> MTTLRAFTCDDLFRFNNINLDPLTETYGIPFYLQYLAHWPEYFIVAEAPGGELMGYIMGKAEGSVAREEWHGHVTALSVAPEFRRLGLAAKLMELLEEISERKGGFFVDLFVRVSNQVAVNMYKQLGYSVYRTVIEYYSASNGEPDEDAYDMRKALSRDTEKK;> MATRGHVQDPNDRRLRPIYDYLDNGNNKMAIQQADKLLKKHKDLHCAKVLKAIGLQRTGKQEEAFTLAQEVAALEPTDDNSLQALTILYREMHRPELVTKLYEAAVKKVPNSEEYHSHLFMAYARVGEYKKMQQAGMALYKIVPKNPYYFWSVMSLIMQSISAQDENLSKTMFLPLAERMVEKMVKEDKIEAEAEVELYYMILERLGKYQEALDVIRGKLGEKLTSEIQSRENKCMAMYKKLSRWPECNALSRRLLLKNSDDWQFYLTYFDSVFRLIEEAWSPPAEGEHSLEGEVHYSAEKAVKFIEDRITEESKSSRHLRGPHLAKLELIRRLRSQGCNDEYKLGDPEELMFQYFKKFGDKPCCFTDLKVFVDLLPATQCTKFINQLLGVVPLSTPTEDKLALPADIRALQQHLCVVQLTRLLGLYHTMDKNQKLSVVRELMLRYQHGLEFGKTCLKTELQFSDYYCLLAVHALIDVWRETGDETTVWQALTLLEEGLTHSPSNAQFKLLLVRIYCMLGAFEPVVDLYSSLDAKHIQHDTIGYLLTRYAESLGQYAAASQSCNFALRFFHSNQKDTSEYIIQAYKYGAFEKIPEFIAFRNRLNNSLHFAQVRTERMLLDLLLEANISTSLAESIKSMNLRPEEDDIPWEDLRDNRDLNVFFSWDPKDRDVSEEHKKLSLEEETLWLRIRSLTLRLISGLPSLNHPVEPKNSEKTAENGVSSRIDILRLLLQQLEATLETGKRFIEKDIQYPFLGPVPTRMGGFFNSGCSQCQISSFYLVNDIYELDTSGLEDTMEIQERIENSFKSLLDQLKDVFSKCKGDLLEVKDGNLKTHPTLLENLVFFVETISVILWVSSYCESVLRPYKLNLQKKKKKKKETSIIMPPVFTSFQDYVTGLQ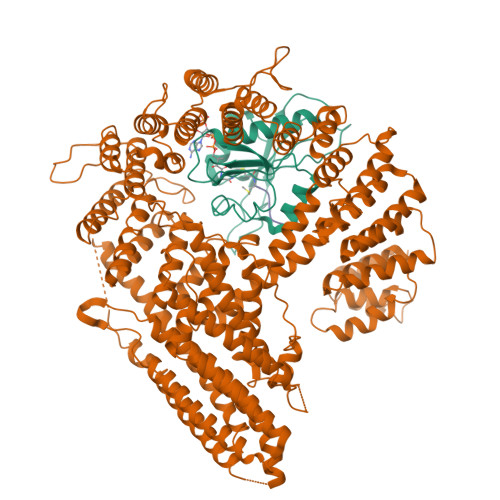TLISNVVDHIKGLETHLIALKLEELILEDTSLSPEERKFSKTVQGKVQSSYLHSLLEMGELLKKRLETTKKLKI;> MDVFM> MGSSHHHHHHSSGLVPRSHMSDQEAKPSTEDLGDKKEGEYIKLKVIGQDSSEIHFKVKMTTHLKKLKESYCQRQGVPMNSLRFLFEGQRIADNHTPK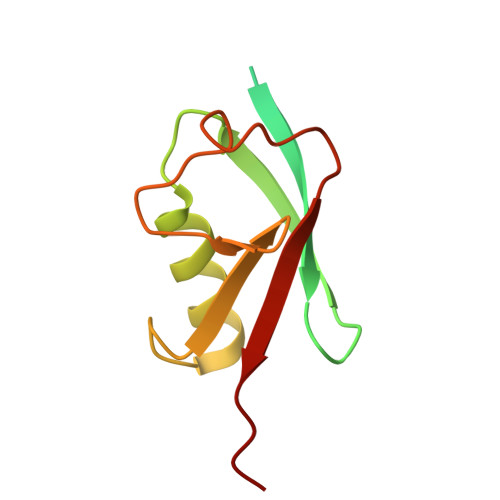ELGMEEEDVIEVYQEQCG>[2x]GAMDSPLQSTLSSAASPSQAYETYIENGLICLKHKIRNIEKKKLKLEDYKDRLKSGEHLNPDQLEAVEKYEEVLHNLEFAKELQKTFSGLSLDLLKAQKKAQRREHMLKLEAEKKKLRTILQVQYV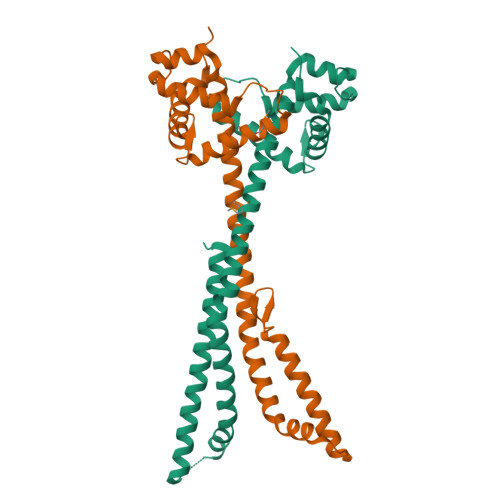LQNLTQEHVQKDFKGGLNGAVYLPSKELDYLIKFSKLTCPERNESLSVEDQMEQSSLYFWDLLEGSEKAVVGTTYKHLKDLLSKLLNSGYFESIPVPKNAKEKEVPLEEEMLIQSEKKTQLSKTESVK> MLSRRYAAKSFVEWYYRQINENKPVASGYVNNNATYTKAGHPPADITINGRVVATPEEWDTMLKEQRAQHNTSSSSTLPIGRKPVRYDVDCFDVHVINADYRFAAPQRMIEQHAPTDGVRMMMALTVS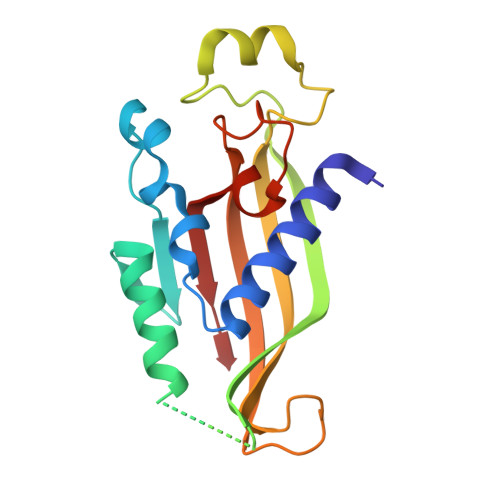GSVYFGASPRSTDDYVIKQHFNDVFILVPNWDVLEKPGARSARKYLIASHKYRAY>DYKDDDDKQNALSLAQTKHSCMALKAEDGEGCTCKQTKRYGQPECCCMGLIVSQLPTNLTADVGYLYLHNTSISVITPNFFDKFPSIRELEIDNSAHLEHIDGSSLSVLSKLRKLSVVKCPNLREISGKLLVNNTRIQNVILKNNGLATMPSLRMTDAHHVLLDRIDLSGNKIKFISDSKVRNVKARTVVLSENKLIEISGYAFTESQFLKLKLNNNPDLRSLSVDAFKNMAGLQTLDLSHTSIDTLPINGLKKLKTLILNDVPTLKSLPSVLSFTDLETAHFTYPHHCCLFKYVDDVTMNDNGKYQRNAKEIHKRICDKREQQKVARRRKRETSGIDFLDMLLKEWTDNSTYTGPDDADDDELPPFVEIGAEPCQSIGEEVQKYYSNITCYPQPDALNPCENIVGYPFLRIAVWVVCLAAIVGNIIVWALLGIVYEKRMRMHYLYMINMSVADMVTGIYLAVLAIADAKMSDEYYRHAVWWQTGWGCRAAGFLAVFASELGIISMFLIAF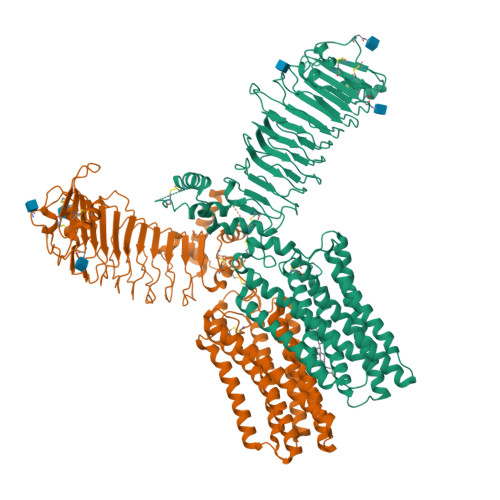EMSYNTRQSFRGRRLSPKVGVLLMIGGWLFAIIMAILPWFDVSSYSESSVCLPLRAATIFDKSYLIFGLSFNFLAFAAMALSYGFIVKMLKENETREEDRALITKMTVLVVTDLICWFPTLFFGFTATIGFPLLSLSSAKFVLVFFFPINAFANPFLYVFFTEVIQHRVRSKTLPVIRRAAADYKDDDDK[2x]> MASKYAVKLKTDFDNPRWIKRHKHMFDFLDINGNGKITLDEIVSKASDDICAKLEATPEQTKRHQVCVEAFFRGCGMEYGKEIAFPQFLDGWKQLATSELKKWARNEPTLIREWGDAVFDIFD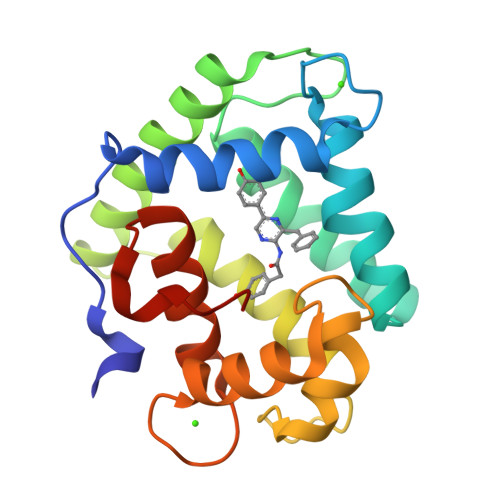KDGSGTITLDEWKAYGKISGISPSQEDCEATFRHCDLDNSGDLDVDEMTRQHLGFWYTLDPEADGLYGNGVP(2R)-2-[(2R,3R,4R,5S,6R)-3-acetamido-2,5-bis(oxidanyl)-6-(phosphonooxymethyl)oxan-4-yl]oxypropanoic acid | C11 H20 N O11 P 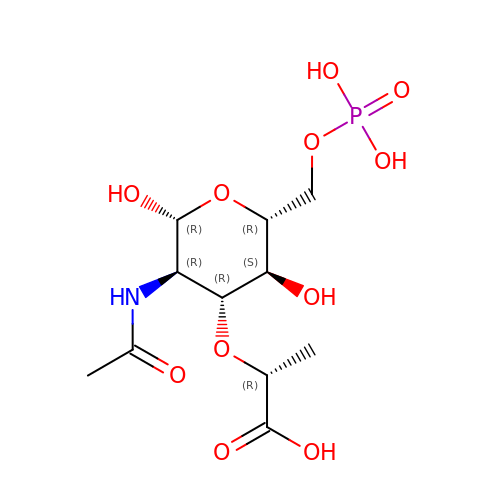| NMEMTQKUEVNSPV-YVNCZSHWSA-N Fucoidanases (EC 3.2.1.–) catalyze the hydrolysis of glycosidic bonds between fucose residues in fucoidans. Fucoidans are a compositionally and structurally diverse class of fucose-containing sulfated polysaccharides that are primarily found in brown seaweeds. Here, the structural characterization of a novel endo-α(1,4)-fucoidanase, Mef1, from the marine bacterium Muricauda eckloniae is presented, showing sequence similarity to members of glycoside hydrolase family 107. Using carbohydrate polyacrylamide gel electrophoresis and nuclear magnetic resonance analyses, it is shown that the fucoidanase Mef1 catalyzes the cleavage of α(1,4)-linkages between fucose residues sulfated on C2 in the structure [-3)-α-l-Fucp2S-(1,4)-α-l-Fucp2S-(1-] n in fucoidan from Fucus evanescens.

By crystal structure determination of Mef1 at 1.8 Å resolution, a single-domain organization comprising a (β/α)8-barrel domain was determined. The amino acids in the groove are largely positively charged, as is especially evident for Arg35, and are likely to assist with the binding and positioning of the largely negatively charged sulfated fucoidan polysaccharide. CAPSO, which is normally used as a buffer, is a small, sulfated molecule and the sulfate group of CAPSO 1 is coordinated in the Mef1 crystal primarily through Arg35, while the EG site is close to a small α-helical structure stabilized by Ca1.

> MKQQLITIIFALGILNISAQTSSDSKWLSGSWGVRLIVEGGVELDKASSYSDWVKGAQNIVDNLPTVGHVFTNFTHRAHGYWFTLRENPYVDVAKEIHPEFVPSLENEKIILDVIDILHKGGKKVILYIATDGPSARSGTRNNAEYKAAWENYYNAKFDGDEGLAYRTLCKGYIERFKGLADGYWLDHVGGIAGELTDFIDMIREVDPSVMIASNGIVENESSNKSKYFKDENGDDLEVDSDGTNDPDGRKYKIRSFNLNGSYVDFTSGHPTPLAWGAPPNSWAYEEFTFPEIVDAMASYDPVKHTIKHAWMPMRMKWTSPRANLMFDVEQAYRFVRTLTDGGCAITWGNTQTNGSMTKEEMDIMKEVDRRLRMRPMPDYIPYKRPAGAKLVGETKTKD(1R,4S,5R)-1,4,5-trihydroxy-3-[(5-methyl-1-benzothiophen-2-yl)methoxy]cyclohex-2-ene-1-carboxylic 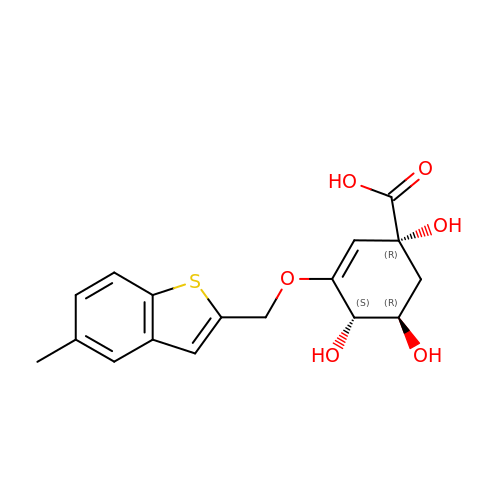acid | C17 H18 O6 S | BNUWPGVZRDEWEX-ISTRZQFTSA-N> MSLKMETGKLLMELSNLDGPSGYETNVVSYIKSVIEPFVDEAKTTRHGSLIGYKKGKGIGKLAFFAHVDEIGFVVSKVEGQFARLEPVGGVDPKVVYASKVRIYTKNGIERGVIGMLAPHLQDSESRKKVPTYDEIFVDLSLCERGVRVGDIAVIDQTAFETNGKVVGKALDNRASCGVLVKV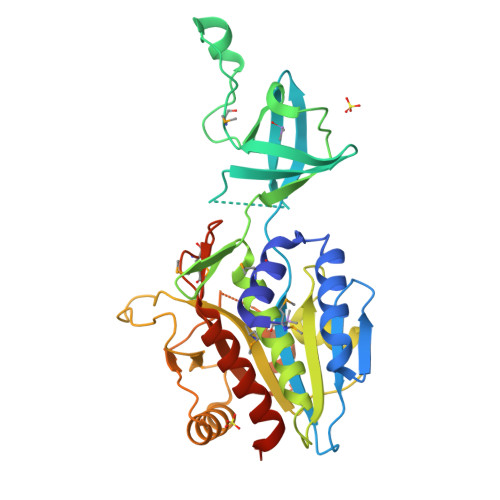LEFLKRYDHPWDVYVVFSVQEETGCLGALTGAYEINPDAAIVMDVTFASEPPFSDHIELGKGPVIGLGPVVDRNLVQKIIEIAKKHNVSLQEEAVGGRSGTETDFVQLVRNGVRTSLISIPLKYMHTPVEMVDPRDVEELARLLSLVAVELEVEGGSHHHHHH> XMHLNPAEKEKLQIFLASELLLRRKARGLKLNYPEAVAIITSFIMEGARDGKTVAMLMEEGKHVLTRDDVMEGVPEMIDDIQAEATFPDGTKLVTVHNPIS;> NYIVPGEYRVAEGEIEINAGREKTTIRVSNTGDRPIQVGSHIHFVEVNKELLFDRAEGIGRRLNIPSGTAARFEPGEEMEVELTELGGNREVFGISDLTNGSVDNKELILQRAKELGYKGVE;> MKINRQQYAESYGPTVGDEVRLADTDLWIEVEKDYTTYGDEVNFGGGKVLREGMGENGTYTRTENVLDLLLTNALILDYTGIYKADIGVKDGYIVGIGKGGNPDIMDGVTPNMIVGTATEVIAAEGKIVTAGGIDTHVHFINPDQVDVALANGITTLFGGGTGPAEGSKATTVTPGPWNIEKMLKSTEGLPINVGILGKGHGSSIAPIMEQIDAGAAGLKIHEDWGATPASIDRSLTVADEADVQVAIHSDTLNEAGFLEDTLRAINGRVIHSFHVEGAGGGHAPDIMAMAGHPNVLPSSTNPTRPFTVNTIDEHLDMLMVCHHLKQNIPEDVAFADSRIRPETIAAEDILHDLGIISMMSTDALAMGRAGEMVLRTWQTADKMKKQRGPLAEEKNGSDNFRLKRYVSKYTINPAIAQGIAHEVGSIEEGKFADLV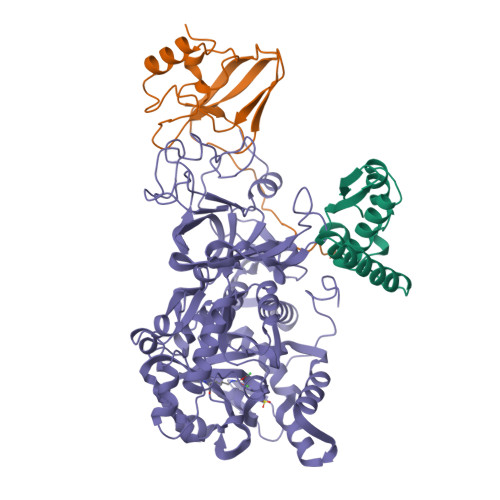LWEPKFFGVKADRVIKGGIIAYAQIGDPSASIPTPQPVMGRRMYGTVGDLIHDTNITFMSKSSIQQGVPAKLGLKRRIGTVKNCRNIGKKDMKWNDVTTDIDINPETYEVKVDGEVLTCEPVKELPMAQRYFLF> GMGFTIDIKSFLKPGEKTYTQRCRLFVGNLPTDITEEDFKRLFERYGEPSEVFINRDRGFGFIRLESRTLAEIAKAELDGTILKSRPLRIRFATHGAALTVKNLSPVVSNELLEQAFSQFGPVEKAVVVVDDRGRATGKGFVEFAAKPPARKAL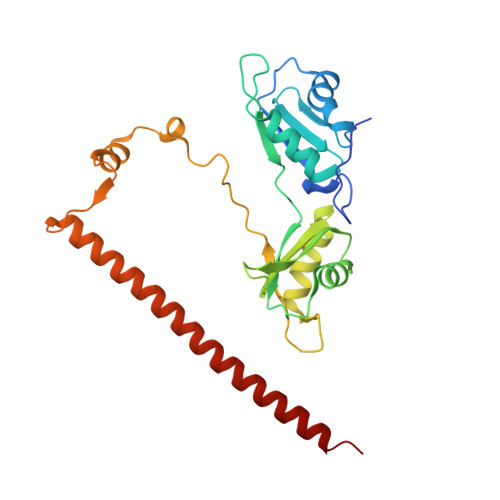ERCGDGAFLLTTTPRPVIVEPMEQFDDEDGLPEKLMQKTQQYHKEREQPPRFAQPGTFEFEYASRWKALDEMEKQQREQVDRNIREAKEKLEAEMEAARHEHQLMLM> MAFSARFPLWLLLGVVLLASVSASFAHSGHSGGEAEDESEESRAQNNPYLFRSNKFLTLFKNQHGS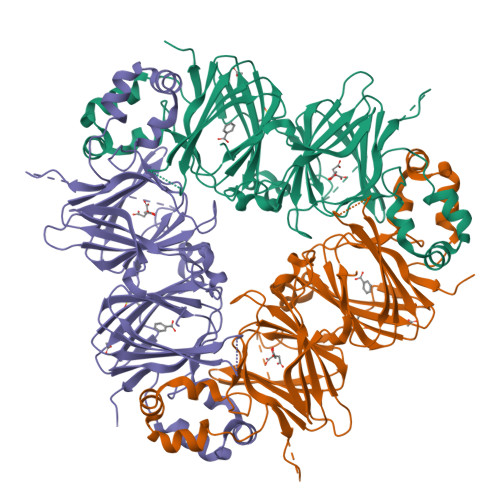LRLLQRFNEDTEKLENLRDYRVLEYCSKPNTLLLPHHSDSDLLVLVLEGQAILVLVNPDGRDTYKLDQGDAIKIQAGTPFYLINPDNNQNLRILKFAITFRRPGTVEDFFLSSTKRLPSYLSAFSKNFLEASYDSPYDEIEQTLLQEEQEGVIVKMPKDQIQEISKHAQSSSRKTLSSQDKPFNLRSRDPIYSNNYGKLYEITPEKNSQLRDLDILLNCLQMNEGALFVPHYNSRATVILVANEGRAEVELVGLEQQQQQGLESMQLRRYAATLSEGDIIVIPSSFPVALKAASDLNMVGIGVNAENNERNFLAGHKENVIRQIPRQVSDLTFPGSGEEVEELLENQKESYFVDGQPRHIDAGGKARRAHLPNLFRTFY> GHMSSTPSNQNIIPIIKKESIVSLFEKGIRQDGRKLTDYRPLSITLDYAKKADGSALVKLGTTMVLAGTKLEIDKPYEDTPNQGNLIVNVELLPLAYETFEPGPPDENAIELARVVDRSLRDSKALDLTKLVIEPGKSVWTVWLDVYVLDYGGNVLDACTLASVAALYNTKVYKVEQHSNGISVNKNEVVGKLPLNYPVVTISVAKVDKYLVVDPDLDEESIMDAKISFSYTPDLKIVGIQKSGKGSMSLQDIDQAENTARSTAVKLLEELKKHLGI;> GHMREMLQVERPKLILDDGKRTDGRKPDELRSIKIELGVLKNADGSAIFEMGNTKAIAAVYGPKEMHPRHLSLPDRAVLRVRYHMTPFSTDERKNPAPSRREIELSKVIREALESAVLVELFPRTAIDVFTEILQADAGSRLVSLMAASLALADAGIPMRDLIAGVAVGKADGVIILDLNETEAMWGEADMPIAMMPSLNQVTLFQLNGSMTPDEFRQAFDLAVKGINIIYNLEREALKSKYVEFKEEGV;> GHMNMSQSQEIVLQPRSIVVPGELL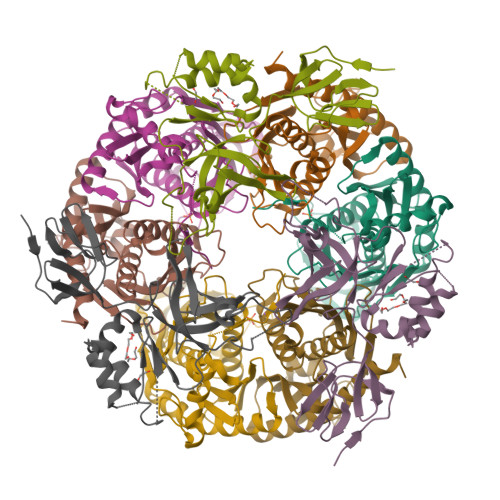AEGEFQIPWSPYILKINSKYYSTVVGLFDVKDTQFEVIPLEGSFYYPKINDIVIGLVEDVEIYGWVVDIKAPYKAYLPASNLLGRSINVGEDLRRYLDVGDYVIARIENFDRSIDPVLSVKGKDLGRVSNGIVIDIMPVKVPRVIGKNKSMYETLTSKSGCSIFVANNGRIWATCPSRFSEEILIEAIRKIENESHIKGLTDRIKQFIEEKLGERNASSGETKTNS> MSHHHHHHSMAALALWAKSGNPFHPLLAHMLDTAAVALAVLRMEPPRTRALYAEDWGLPEEGALAWAAALVGL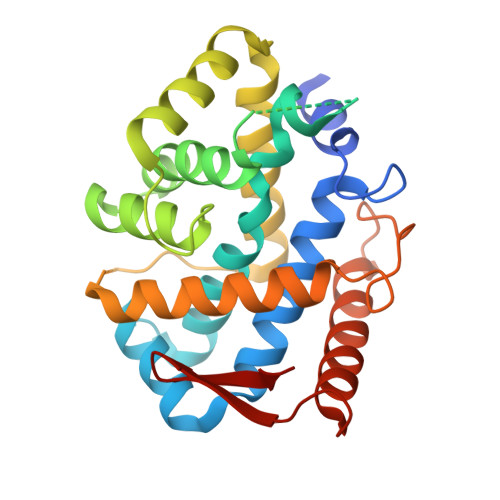HDLGKASPVFQAGWEEGKERVQRAGLPFGELLDWVAHGVFTELFLRRLLKEKGLPERAANDLAAALGAHHGFPANAEEKSRARRHLRTEDPLWKEARRWLLEEVFRRLGAPLPPSQGNGEARPEAVLRVMALASFADWVASDPSLFPYGRDPRRGDYLKEALRLAQEALNRLGWPAFAKAQRREFGELFPYI> MENGKRDRQDMEVNTTPRKPRVLLAASGSVAAIKFGNLCHCFTEWAEVRAVVTKSSLHFLDKLSLPQEVTLYTDEDEWSSWNKIGDPVLHIELRRWADVLVIAPLSANTLGKIAGGLCDNLLTCIIRAWDYTKPLFVAPAMNTLMWNNPFTERHLLSLDELGITLIPPIKKRLACGDYGNGAMAEPSLIY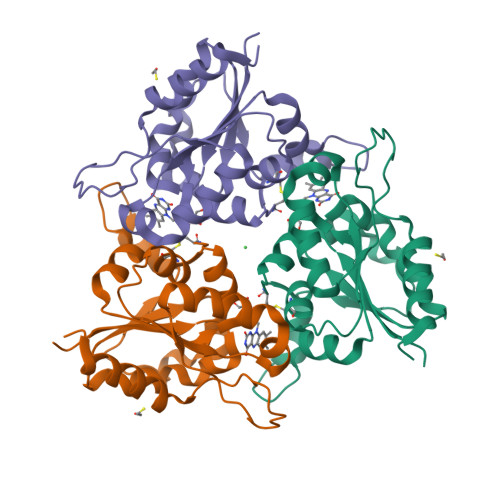STVRLFWESQAHQQTGGTS>[8x]GAMAPADIVKNLKDNMTILEKQDISDKKAEKASEEVSKSLLSMKEILYGTNEKEPQTEAVAQLAQELYNSGLLSTLVADLQLIDFEGKKDVAQIFNDILRRQIGTRTPTVEYLCTQQNILFMLLKGYE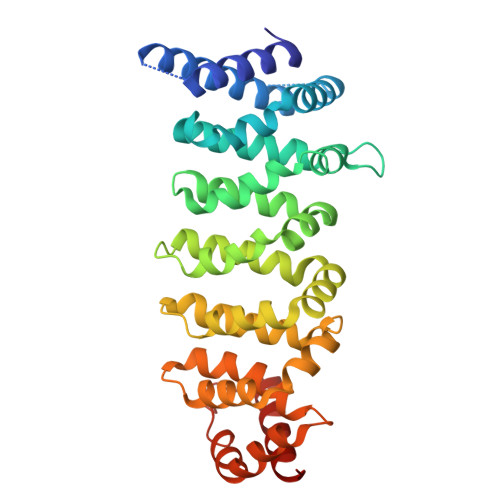SPDIALNCGIMLRECIRHEPLAKITLCSEQFYDFFRYVEMSTFDIASDAFATFKDLLTRHKVLSAEFLEQHYDRFFSEYEKLLHSENYVTKRQSLKLLGELLLDRHNFTIMTKYISKPENLKLMMNLLRDKSRNIQFEAFHVFKVFVANPNKTPPILDILLKNQTKLIEFLSKFQNDRAEDEQFSDEKTYLIKQIRDLK>[16x]GAMAKETTPVALSFHDLHQLTRAAVERAQQLQVPVVVSIVDAHGTETVTWRMPDALLVSSELAPKKAWTAVAMKTATHELSDV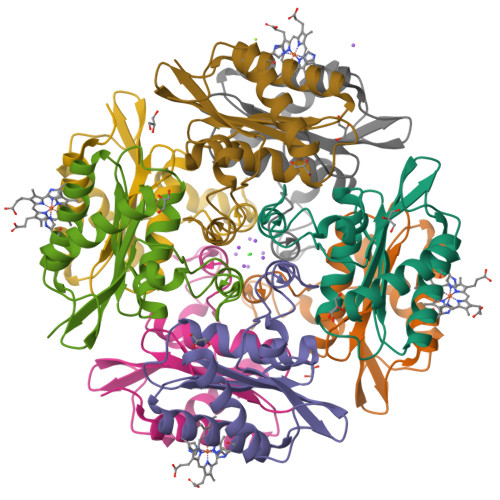VQPGAALYGLESHLQGKVVTFGGGYALWRDGILIGGLGISGGSVEQDMDIAQTAIAAINVGTHQ1-(2-methyl-4-phenyl-pyrimidin-5-yl)-3-naphthalen-1-yl-urea 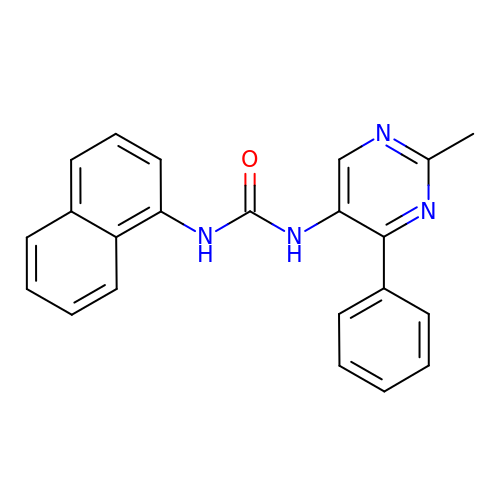| C22 H18 N4 O | QTGKTWMSCVUXHK-UHFFFAOYSA-N N-(1-BENZYL-3-{[3-(1,3-DIOXO-1,3-DIHYDRO-ISOINDOL-2-YL)-PROPIONYL]-[2-(HEXAHYDRO-BENZO[1,3]DIOXOL-5-YL)-ETHYL]-AMINO}-2-HYDROXY-PROPYL)-4-BENZYLOXY-3,5-DIMETHOXY-BENZAMIDE | C46 H51 N3 O10 | 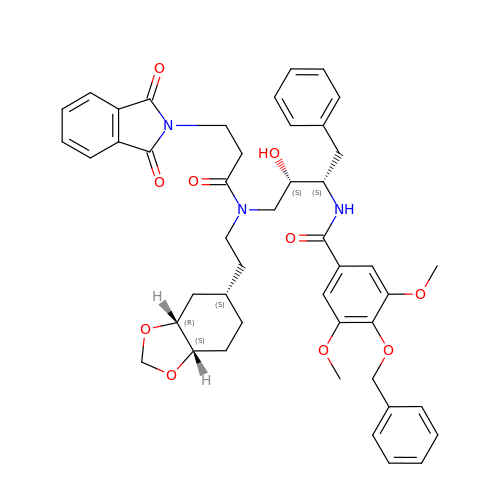PJQGNNQTZMYXOB-HAMMGQCISA-N>[2x]SNILEMTKNYYDRSVSPVEYAYFDQSQNMRAINWNKIVDEKDLEVWNRVTQNFWLPENIPVSNDLPSWNELDDDWQQLITRTFTGLTLLDTVQSSIGDVAQIKNSLTEQEQVIYANFAFMVGVHARSYGTIFSTLCTSEQIEEA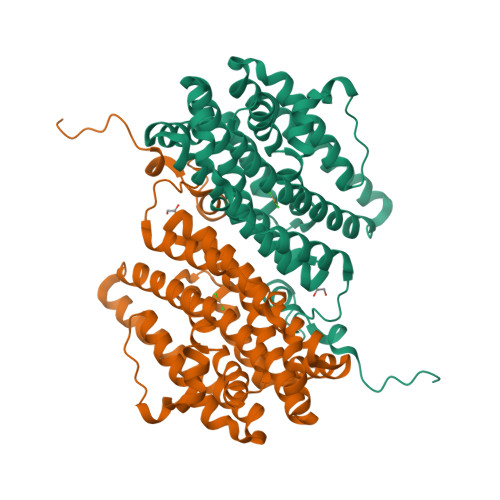HEWVVDNEALQARPKALIPFYTADDPLKSKIAAALMPGFLLYGGFYLPFYLSARGKLPNTSDIIRLILRDKVIHNFYSGYKYQLKVAKLSPEKQAEMKQFVFDLLDKMIGLEKTYLHQLYDGFGLADEAIRFSLYNAGKFLQNLGYESPFTKEETRIAPEVFAQLSARADENHDFFSGSGSSYIIGTSEETLDEDWDF>[4x]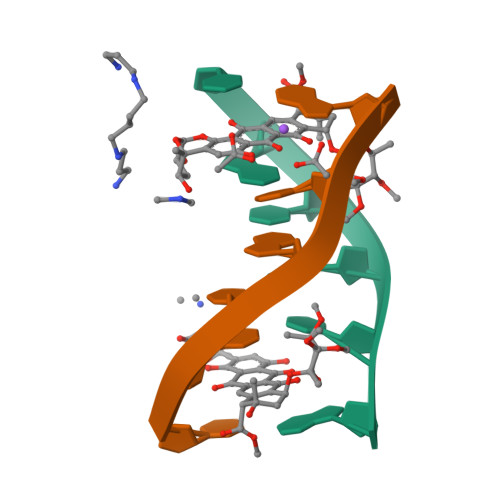TGTACA>MRGSPHHHHHHGSAKNVVLDHAGNLDDFVAMVLLASNTEKVRLIGALCTDADCFVENGFNVTGKIMCLMHNNMNLPLFPIGKSAATAVNPFPKEWRCLAKNMDDMPILNIPENVELWDKIKAENEKYEGQQLLADLVMNSEEKVTICVTGPLSNVAWCIDKYGEKFTSKVEECVIMGGAVDVRGNVFLPSTDGTAEWNIYWDPASAKTVFGCPGLRRIMFSLDSTNTVPVRSPYVQRFGEQTNFLLSILVGTMWAMCTHCELLRDGDGYY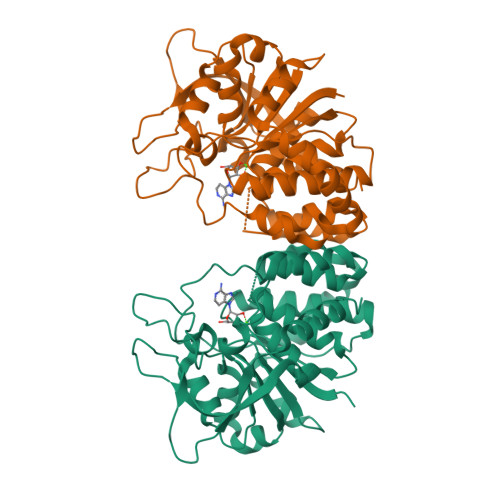AWDALTAAYVVDQKVANVDPVPIDVVVDKQPNEGATVRTDAENYPLTFVARNPEAEFFLDMLLRSARAC[2x]>[2x]MNQLEMKKLAAQAALQYVKADRIVGVGSGSTVNCFIEALGTIKDKIQGAVAASKESEELLRKQGIEVFNAND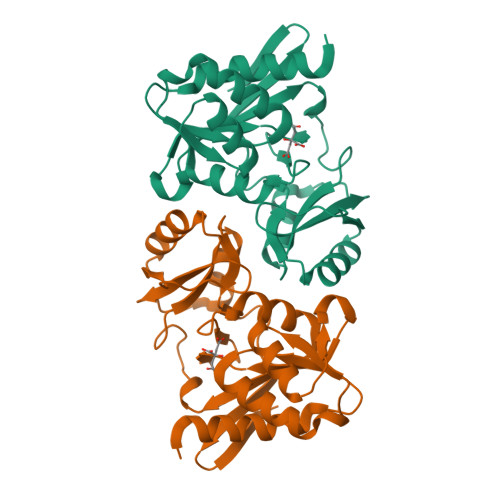VSSLDIYVDGADEINPQKMMIKGGGAALTREKIVAALAKKFICIVDSSKQVDVLGSTFPLPVEVIPMARSQVGRKLAALGGSPEYREGVVTDNGNVILDVHNFSILNPVEIEKELNNVAGVVTNGIFALRGADVVIVGTPEGAKVID>[2x]MVSVSEIRKAQRAEGPATILAIGTANPANCVEQSTYPDFYFKITNSEHKTELKEKFQRMCDKSMIKRRYMYLTEEILKENPNVCEYMAPSLDARQDMVVVEVPRLGKEAAVKAIKEWGQPKSKITHLIVCTTSGVDMPGADYQLTKLLGLRPYVKRYMMYQQGCFA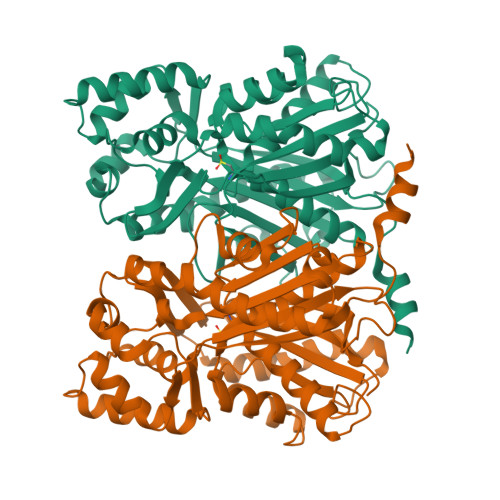GGTVLRLAKDLAENNKGARVLVVCSEVTAVTFRGPSDTHLDSLVGQALFGDGAAALIVGSDPVPEIEKPIFEMVWTAQTIAPDSEGAIDFHLREAGLTFHLLKDVPGIVSKNITKALVEAFEPLGISDYNSIFWIAHPGGPAILDQVEQKLALKPEKMNATREVLSEYGNMSSACVLFILDEMRKKSTQNGLKTTGEGLEWGVLFGFGPGLTIETVVLRSVAI>[4x]MDAQYDISFADVEKAHINIRDSIHLTPVLTSSILNQLTGRNLFFKCELFQKTGSFKIRGALNAVRSLVPDALERKPKAVVTHSSGNHGQALTYAAKLEGIPAYIVVPQTAPDCKKLAIQAYGASIVYCEPSDESRENVAKRVTEETEGIMVHPNQEPAVIAGQGTIALEVLNQVPLVDALVVPVGGGGMLAGIAITVKALKPSVKVYAAEPSNADDCYQSKLKGKLMPNLYPPETIADGVKSSIGLNTWPIIRDLVDDIFTVTEDEIKCATQLVWERMKLLIEPTAGVGVAAVLSQHFQTVSPEVKNICIVLSGGNVDLTSSITWVKQAERPASYQSVSVHHHHHH

Human serine racemase (hSR) catalyses racemisation of L-serine to D-serine, the latter of which is a co-agonist of the NMDA subtype of glutamate receptors that are important in synaptic plasticity, learning and memory. In mammals, D-serine is synthesised by a pyridoxal-5′-phosphate (PLP)-containing enzyme serine racemase (SR). The first mammalian structures of SR, published in 201031, revealed a dimeric structure with each subunit consisting of a small domain (residues 78–153) and a large domain (residues 4–67 and 156–316). The roles of Ser 84 and Lys 56 as the Si and Re-face acid/bases in the catalytic cycle of hSR are generally accepted.

In contrast, in ‘open’ hSR structures, Tyr121 sits in the core of the small domain with its hydroxyl contacting the key catalytic residue Ser84. Analysis of 600 fragment-soaked hSR crystals revealed 44 interesting binding events, of which twelve had displaced Tyr 121 from the core of the small domain in at least one of the four subunits in the asymmetric unit. One of these is a 1.53 Å crystal structure of hSR bound to compound 1-x0495 (Fig. 3a, A-subunit; Supplementary Table 4 for XChem ligand structures). The difference between the conformations of the A- and C-subunits can be seen when there is no compound bound to either subunit. Interestingly, of the four subunits in the asymmetric unit, subunit C is locked in a slightly different open conformation. and compound 13-x0430, was only observed to bind to the C subunit.>GPGSHLAHPNLDTFTPEELLQQMKELLTENHQLKEAMKLNNQAMKGRFEELSAWTEKQKEERQFFEIQSKEAKERLMALSHE[2x];>GPGSYPSSNTLVEMTLGMKKLKEEMEGVVKELAENNHILERF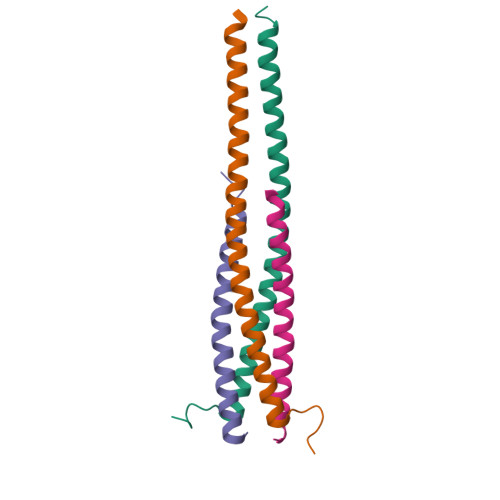GSLTMDGGLRNVDCL[2x]> GAQVSTQKTGAHETSLTASGNSTIHYTNINYYKDAASNSANRQDFTQDPSKFTEPMKDVMIKSLPALNSPTVEECGFSDRVRSITLGNSTITTQECANVVVGYGVWPSYLQDNEATAEDQPTQPDVATCRFYTLDSIQWQKESDGWWWKFPEALKNMGLFGQNMEYHYLGRSGY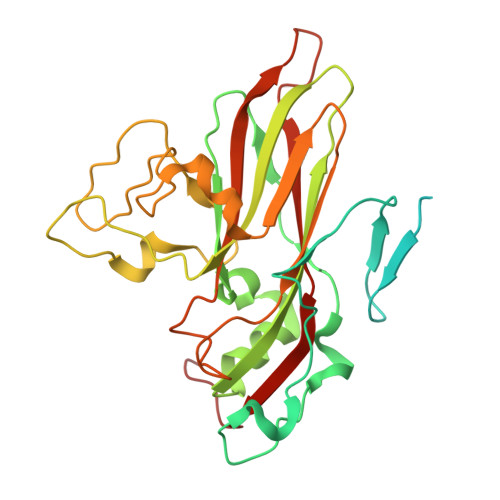TIHVQCNASKFHQGCLLVVCVPEAEMGCSDVEREVVAASLSSEDTAKSFSRTESNGQHTVQTVVYNAGMGVGVGNLTIFPHQWINLRTNNSATIVMPYINSVPMDNMFRHYNFTLMIIPFAKLEYTEQASNYVPITVTVAPMCAEYNGLRLASHQ>MTDMNILDLFLKASLLVKLIMLILIGFSIASWAIIIQRTRILNAAAREAEAFEDKFWSGIELSRLYQESQGKRDNLTGSEQIFYSGFKEFVRLHRANSHAPEAVVEGASRAMRISMNRELENLETHIPFLGTVGSISPYIGLFGTVWGIMHAFIALGAVKQATLQMVAPGIAEALIATAIGLFAAIPAVMAYNRLNQRVNKLELNYDNFMEEFTAILHRQAFTVSESNKG[5x];>[2x]MARARGRGRRDLKSEINIVPLLDVLLVLLLIFMATAPIITQSVEVDLPDATESQAVSSNDNPP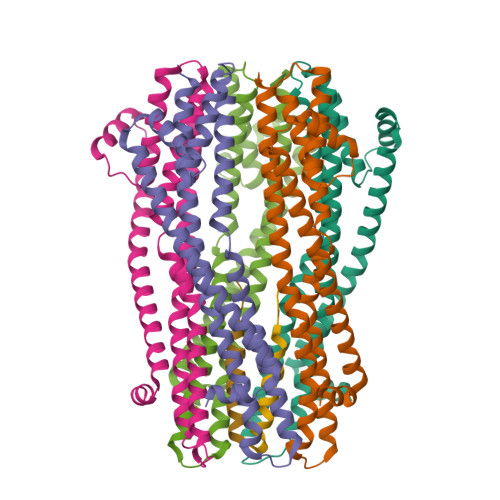VIVEVSGIGQYTVVVEKDRLERLPPEQVVAEVSSRFKANPKTVFLIGGAKDVPYDEIIKALNLLHSAGVKSVGLMTQPI>MEIKRVGSQASGKGPADWFTGTVRIDPLFQA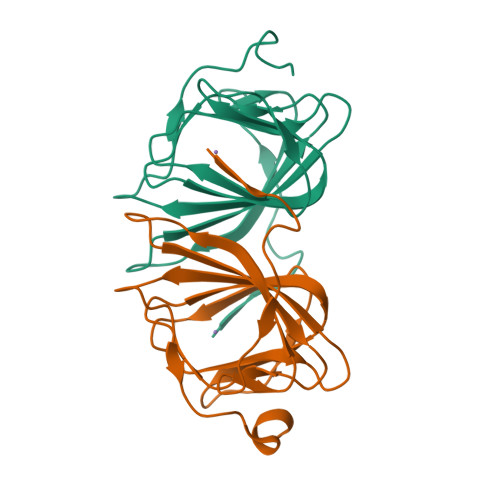PDPALVAGHSTTFEPGARTAWHTHPLGQTLIVTAGCGWAQREGGAVEEIHPGDVVWFSPGEKHWHGAAPTTAMTHLAIHERLDGKAVDWMEHVTDEQYRR[20x]>[2x]MGSSHHHHHHSQDPNSMPDNTIQWDKDADGIVTLTMDDPSGSTNVMNEAYIESMGKAVDRLVAEKDSITGVVVASAKKTFFAGGDVKTMIQARPEDAGDVFNTVETIKRQLRTLETLGKPVVAAINGAALGGGLEIALACHHRIAADVKGSQLGLPEVTLGLLPGGGGVTRTVRMFGIQNAFVSVLAQGTRFKPAKAKEIGLVDELVATVEELVPAAKAWIKEELKANPDGAGVQPWDKKGYKMPGGTPSSPGLAAILPSFPSNLRKQLKGAPMPAPRAILAAAVEGAQVDFDTASRIESRYFASLVTGQVAKNMMQAFFFDLQAIN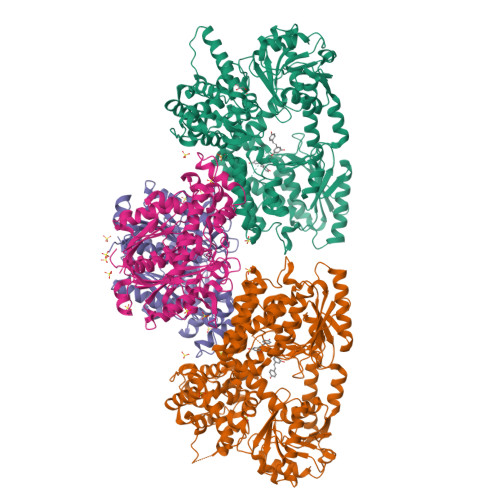AGGSRPEGIGKTPIKRIGVLGAGMMGAGIAYVSAKAGYEVVLKDVSLEAAAKGKGYSEKLEAKALERGRTTQERSDALLARITPTADAADFKGVDFVIEAVFENQELKHKVFGEIEDIVEPNAILGSNTSTLPITGLATGVKRQEDFIGIHFFSPVDKMPLVEIIKGEKTSDEALARVFDYTLAIGKTPIVVNDSRGFFTSRVIGTFVNEALAMLGEGVEPASIEQAGSQAGYPAPPLQLSDELNLELMHKIAVATRKGVEDAGGTYQPHPAEAVVEKMIELGRSGRLKGAGFYEYADGKRSGLWPGLRETFKSGSSQPPLQDMIDRMLFAEALETQKCLDEGVLTSTADANIGSIMGIGFPPWTGGSAQFIVGYSGPAGTGKAAFVARARELAAAYGDRFLPPESLLS;>MSEEAFIYEAIRTPRGKQKNGSLHEVKPLSLVVGLIDELRKRHPDLDENLISDVILGCVSPVGDQGGDIARAAVLASGMPVTSGGVQLNRFCASGLEAVNTAAQKVRSGWDDLVLAGGVESMSRVPMGSDGGAMGLDPATNYDVMFVPQSIGADLIATIEGFSREDVDAYALRSQQKAAEAWSGGYFAKSVVPVRDQNGLLILDHDEHMRPDTTKEGLAKLKPAFEGLAALGGFDDVALQKYHWVEKINHVHTGGNSSGIVDGAALVMIGSAAAGKLQGLTPRARIVATATSGADPVIMLTGPTPATRKVLDRAGLTVDDIDLFELNEAFASVVLKFQKDLNIPDEKLNVNGGAIAMGHPLGATGAMILGTMVDELERRNARRALITLCIGGGMGVATIIERV[2x]Here we use a robust deep learning pipeline to design complex folds and soluble analogues of integral membrane proteins. Unique membrane topologies, such as those from G-protein-coupled receptors, are not found in the soluble proteome, and we demonstrate that their structural features can be recapitulated in solution. Biophysical analyses demonstrate the high thermal stability of the designs, and experimental structures show remarkable design accuracy. The soluble analogues were functionalized with native structural motifs, as a proof of concept for bringing membrane protein functions to the soluble proteome, potentially enabling new approaches in drug discovery.

Finally, we attempted to design a TBF, a challenging protein topology that is of paramount importance in biology, as its structure is highly proficient in supporting enzymatic active sites, making it an ideal candidate for the design of enzymes with new catalytic functions. The TBF comprises eight parallel-paired β-strands, each separated by an α-helix, resulting in long-range interactions between the β-strands. The TBF has been a longstanding challenge in protein design, and it is only very recently that several studies have successfully designed this fold. Previous TBF design strategies imposed symmetry and parametric restraints at both the structural and sequence levels. With our pipeline, we could design TBFs without any constraints, allowing greater structural and sequence diversity and even asymmetry, which could potentially accommodate more complex enzymatic sites. We experimentally assessed 25 designs, five of which were monomeric, folded and highly thermostable in solution. To confirm the accuracy of our design, we solved a crystal structure of TBF_24 at 1.34 Å resolution. Our asymmetric design showed noticeable structural deviations from the initial symmetric template, with an overall backbone r.m.s.d.Cα (root mean square deviation computed over the Cα atoms of the backbone) of 2.06 Å. Comparison of the X-ray structure with the designed model showed the r.m.s.d.Cα and full-atom r.m.s.d.fa (root mean square deviation computed over all the atoms in the structure) were 0.80 Å and 2.12 Å, respectively. These structural comparisons demonstrate the remarkable accuracy of our design approach, further underlined by the almost identical side-chain placement in both the core and peripheral regions of the protein.

> MSTIEELIKAAKELKSLGIENIIIEVKSAEDAKKIAAEGFEKILVSGPKTEEGIAMAAAAKAAGAKNIIVTARTAEEALAALATPGVTGVLLTTTAEEAPAALATLKAAGYTNVIFRGPSIEEVKKMIEYGAEKVLISSKDDEEAIKAAAELKAKGVKNIIVATRDIEAAKKAYEAGASSILLVPDGSWG> NPYLFESQRFRSRFRASHGDFRILERFNQRSQLLKGIEKYRVAILELEPQSFVLPHHCDGEAIYVVVKGQGVINIAEQDNKNSFNLQKGDVIRLFAGSNVYLLNKDNNEKLFVYVLAKSVNAPGNLQEYFSAGGQNPESFYRAFSSDILESAFNNPRDKLERLFGQHKEGIIIKASEEQIRAISEHASRSTQQTRGRTQGPFNLMKERPVFESRFGQFFEARPERYEQLRDLDAAVGFMNINQGGMVLPYYNTKSTKLVMVIEGNARFEMACPHLGRQSQSPWSR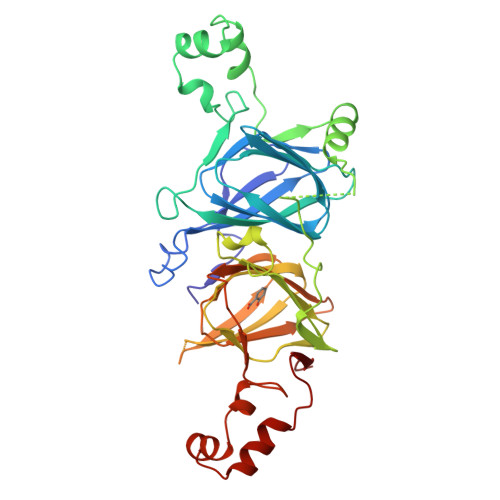GQGREQEREQEQEQEEGDVHYQKIRGNLNVGDVLVIPAGHPITFVATGNSNLRIVGFGVDAENNKKNFLAGKQNIWRNIDREAKELSFSMPGREVEEIFQRQDQSYFVAGPE beta-D-fucofuranose | C6 H12 O5 | 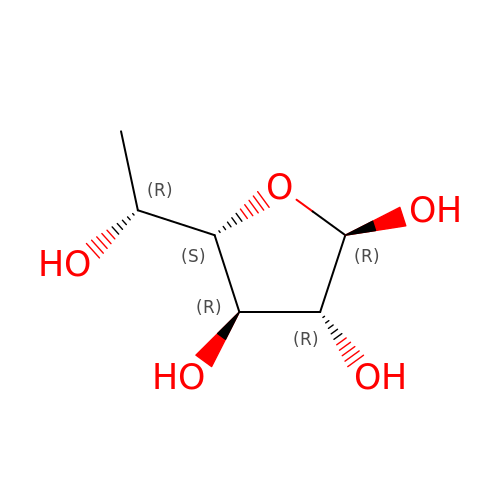AFNUZVCFKQUDBJ-DGPNFKTASA-N>MVNTVNYFKQKLKTEQQIGMWVGLADGYCAEIAANVGYDWLLIDGEHAPNDVRSILAQLQSIAAYPSQAVVRPVSGDVPLIKQLLDIGAQTLLIPMVESAEQAELMVKATRYPPEGIRGVGAALARASRWNNISDYLQTADEQICLLVQVESKKGLDNLDEILNVDGVDGIFIGPADLSAALGYRGNPGHEFVQNIIVQTIQKIRAAGKAAGILSADEKLAKQYLELGT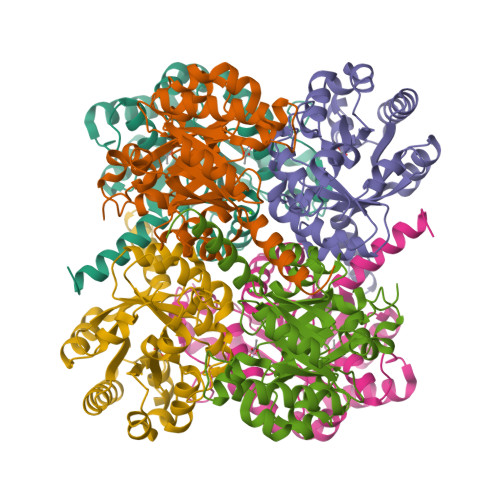EFVAVGVDTSLLMKSMKQLLSKFKNVDGPVSTSPSVY[3x]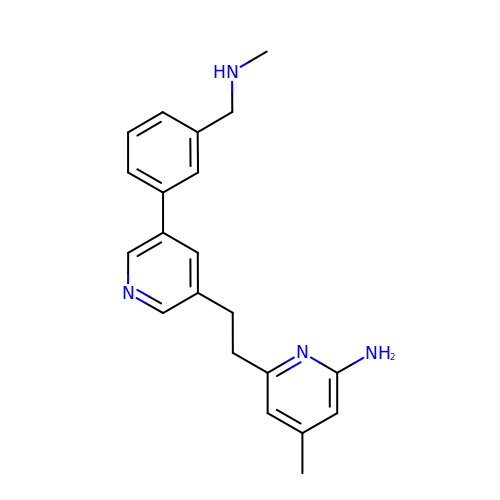4-methyl-6-[2-(5-{3-[(methylamino)methyl]phenyl}pyridin-3-yl)ethyl]pyridin-2-amine | C21 H24 N4 | MGNVQSKYSZRQCR-UHFFFAOYSA-N> LSLMPWFHGKISGQEAVQQLQPPEDGLFLVRESARHPGDYVLCVSFGRDVIHYRVLHRDGHLTI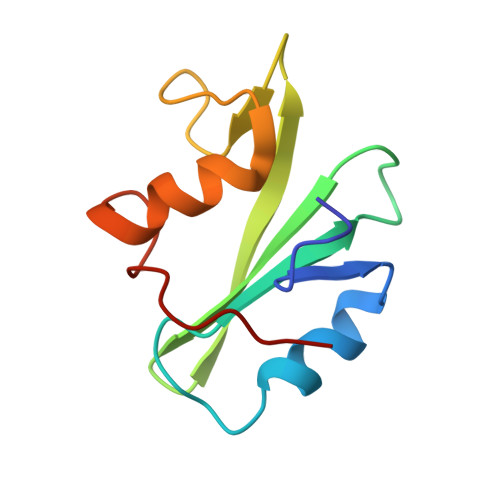DEAVFFCNLMDMVEHYSKDKGAICTKLVRPKRK4,4-dihydroxy-5-oxo-L-norvaline | C5 H9 N O5 | 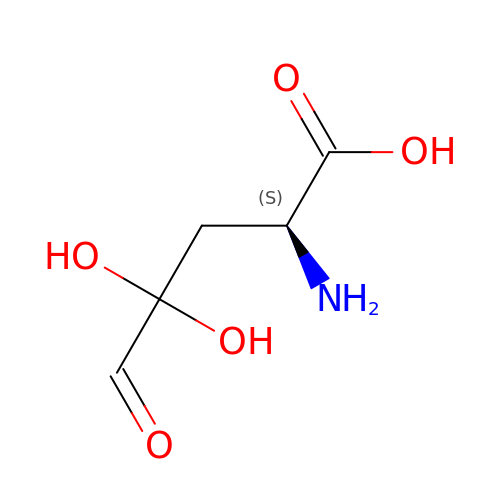NKTBKFGHLWDKLW-VKHMYHEASA-N The GS in H. pylori (Hpy GS) is a critical enzyme that is involved in processing the ammonia released by urease activity, and nitrogen metabolism. GS is an enzyme involved in the biosynthetic reaction producing glutamine from the condensation of glutamate and ammonia. This enzyme is present in all living organisms and is a large homo-oligomeric complex composed of eight, ten, or twelve subunits assembled into two face-to-face rings. Although the structural and sequence information of Hpy GS indicate its relationship with GS I-β due to the presence of a specific 25-amino acid residues (residues 155–179), the adenylation site (NLYDLP) found in similar homologs is replaced in Hpy GS (NLF407KLT), suggesting a lack of the adenylation regulatory mechanism in Hpy GS.

Although a hexamer of Hpy GSapo was present in each asymmetric unit of the crystal, it could be used to generate a dodecamer with 62 symmetry by stacking two hexameric rings face-to-face. In each subunit, N-terminal residues (Met1–Asn7 in subunit A, E, and F; Met1–Gln6 in subunit B, C, and D) and internal residues (Leu408–Gly418 in all subunits) were disordered. Six subunits in the asymmetric unit of Hpy GSapo were almost identical to each other with root-mean-square deviation (r.m.s.d.) values of 0.22–0.27 Å for 474 Cα atoms in residues 8–481. Superposition of Hpy GSapo and Hpy GSsub gave a r.m.s.d. value of 0.50 Å for 473 Cα residues (residues 9–481), and a r.m.s.d. value of 0.50 Å for 4,742 Cα atoms for dodecamer-dodecamer comparisons. The adenylation loops had higher r.m.s.d. values, which may be attributed to the disorder of the loop. These results indicated that Hpy GS does not undergo a large conformational change upon substrate binding. However, the Glu flap in both the Hpy GSapo and Hpy GSsub structures showed a similar closed conformation with little differences. However, the open form of GS was not found in Hpy GS, and the Glu flap was well ordered with a closed conformation in Hpy GSapo in the absence of substrates. This suggests that Hpy GS could exist in either the open or closed form regardless of the presence of substrates.

>MIVRTQNSESKIKEFFEFCKENEVEFVDFRFSDIKGTWNHIAYSFGALTHGMLKEGIPFDASCFKGWQGIEHSDMILTPDLVRYFIDPFSADVSVVVFCDVYDVYKNQPYEKCPRSIAKKALQHLKDSGLGDVAYFGAENEFFIFDSIKIKDASNSQYYEVDSEEGEWNRDRSFENGVNFGHRPGKQGGYMPVPPTDTMMDIRTEIVKVLNQVGLETFVVHHEVAQAQGEVGVKFGDLVEAADNVQKLKYVVKMVAHLNGKTATFMPKPLYGDNGSGMHTHVSVWKNNENLFSGETYKGLSEFALHFLGGVLRHARGLAAFTNASTNSYKRLIPGYEAPSILTYSANNRSASVRIPYGISKNSARFEFRFPDSSSNPYLAFAAILMAGMDGVKNKIDPGEAMDINLFKLTLDEIREKGIKQMPHTLRRSLEEMLADKQYLKESQVFSEEFIQAYQSLKFNAEVFPWESKPHPFEFITTYSC[6x]> MSSAIKEVQGAPVKWVTNWTPEAIRGLVDQEKGLLDPRIYADQSLYELELERVFGRSWLLLGHESHVPETGDFLATYMGEDPVVMVRQKDKSIKVFLNQCRHRGMRICRSDAGNAKAFTCSYHGWAYDIAGKLVNVPFEKEAFCDKKEGDCGFDKAEWGPLQARVATYKGLVFANWDVQAPDLETYLGDARPYMDVMLDRTPAGTVAIGGMQKWVIPCNWKFAAEQFCSDMYHAGTTTHLSGILAGIPPEMD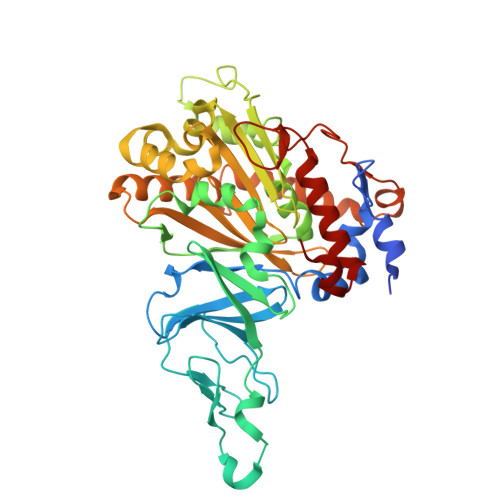LSQAQIPTKGNQFRAAWGGHGSGWYVDEPGSLLAVMGPKVTQYWTEGPAAELAEQRLGHTGMPVRRMVGQHMTIFPTCSFLPTFNNIRIWHPRGPNEIEVWAFTLVDADAPAEIKEEYRRHNIRNFSAGGVFEQDDGENWVEIQKGLRGYKAKSQPLNAQMGLGRSQTGHPDFPGNVGYVYAEEAARGMYHHWMRMMSEPSWATLKP>MAEKPKLHYFNARGRMESTRWLLAAAGVEFEEKFIKSAEDLDKLRNDGYLMFQQVPMAEIDGMKLVQTRAILNYIASKYNLYGKDIKERALIDMYIEGIADLGEMILLLPVCPPEEKDAKLALIKEKIKNRYFPAFEKVLKSHGQDYLVGNKLSRADIHLVELLYYVEELDSSLISSFPLLKALKTRISNLPTVKKFLQPGSPRKPPMDEKSLEE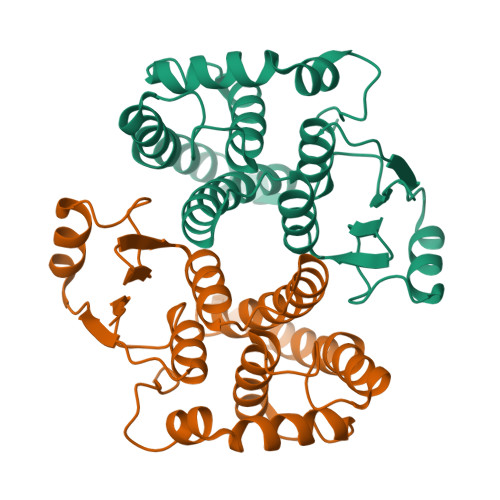ARKIFRF[2x]>[4x]MASVQDVTERKKAEANKALVSREIAHRFKNSMAMVQSIANQTLRNTYDPEQANRL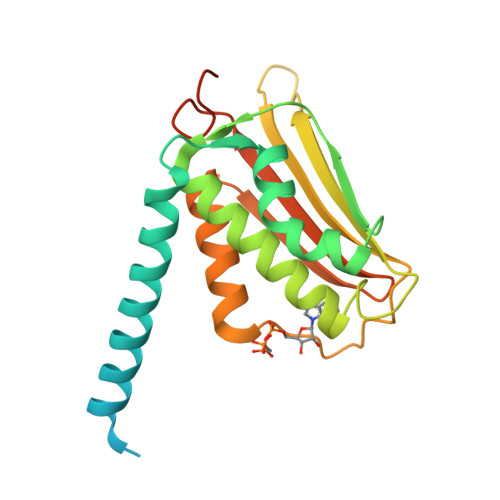FSERLRALSQAHDMLLKENWAGATIQQICATALAPFNSTFANRIHMSGPHLLVSDRVTVALSLAFYELATNAVKYGALSNEKGVINITWAIMEDKGEKKFHMRWAESRGPEVMQPARRGFGQRLLHSVLAEELKAKCDVEFAASGLLIDVLAPITPEVFPGMGHNVPEQRIAHHHHHH> SNAKTESQSHLNTKSDIQYNSAFSQLESDYGAKLGVYAFDTETNKE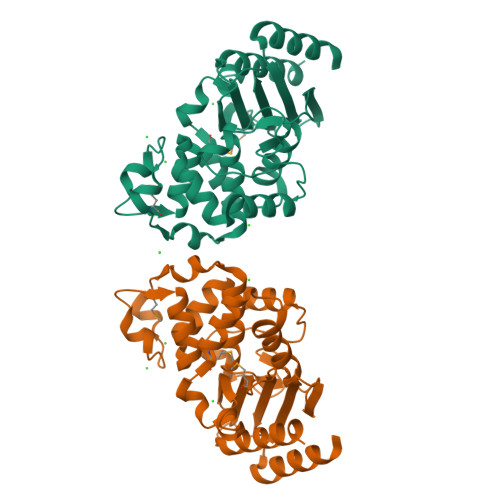VAYRADDRFAYCSTFKALAAGAVLKQDSLEQLKQLVKYKKEDVLSYAPIAKDNVDKGMTIEEICSAAIRFSDNTAANLLLNHIGGPKGFKSALNQLGDSVTQPVHIEPELNEGIPGDIGDTSTPRQLATDLQAYTTGNILTEDKKKILIDWMAGNTTGNTLIRAGAPKSWIVADKSGTGPYGRRNDIAIVMPPNKKPIIIAILSTHDTKEAKYDDKLIAKASKIIFDSFTTTENKE A deazaflavin-dependent nitroreductase (Ddn) from Mycobacterium tuberculosis catalyzes the reduction of nitroimidazoles such as PA-824, resulting in intracellular release of lethal reactive nitrogen species. The N-terminal 30 residues of Ddn are functionally important but are flexible or access multiple conformations, preventing structural characterization of the full-length, enzymatically active enzyme. The split barrel-like fold is characterized by a central six-stranded antiparallel β barrel in a Greek key topology with four α helices: A at the N terminus (the putative helix removed for Ddn structure determination), B after an extended loop between strands β3 and β4, and C and D between strands β5 and β6. The identification of these residues and the lack of classic catalytic residues in the active site suggest that Ddn functions primarily by precisely orienting PA-824 for efficient direct hydride transfer from F420 and potentially through additional transition-state stabilization.

Cocrystals of the NΔ40 construct with oxidized F420 were also obtained in two space groups and were solved by molecular replacement (Holo-1 in C2 at 2.1 Å resolution and Holo-2 in P21 at 1.8 Å resolution, with an rmsd for one chain of 0.3 Å over 109 aligned Cα atoms). The data from both crystals yielded clear difference electron density for the F420 coenzyme, with two glutamate residues in the tail that could be easily positioned. The crystal packing combined with crystallographic symmetry operations reveals the same decameric ring structure in both structures, with five monomers in the ASU of Holo-1 and ten in Holo-2 (two rings per ASU). In structures Holo-1 and Holo-2, F420 binds to a groove on the surface of Ddn through a series of hydrogen bonds and several salt bridges between positive charges on Ddn and the negatively charged phosphate and tail of the coenzyme. The sum of these interactions results in the Re face of F420 being presented for reaction with PA-824. The largest conformational changes between the apo- and F420-bound structures occur near the deazaflavin ring. The loop following strand β3 (residues 76–85) shifts away from the binding site in the presence of coenzyme in order to form the direct contacts to the phosphate and deazaflavin heterocycle outlined above, with the Cα of S78 moving approximately 4 Å in Holo-1 versus Apo-1. In Holo-1 and Holo-2, this loop packs against α helix D (residues 131–139) and generally exhibits lower mobility, indicated by a drop in atomic displacement parameters (ADPs) relative to the apo structures. Modeling was used to visualize the binding mode of PA-824, using the Holo-1 structure with F420 and placing the imidazole group of PA-824 at an appropriate distance from C5 of the flavin ring for hydride transfer (based on observations for other flavin-binding proteins; Fraaije and Mattevi, 2000).

>[5x]GFQKIPVALLTTTGRKTGQPRVNPLYFLRDGGRVIVAASKGGAEKNPMWYLNLKANPKVQVQIKKEVLDLTARDATDEERAEYWPQLVTMYPSYQDYQSWTDRTIPIVVCEP> MSLHEKMQTDYLWVKDHSQADSWAKARTHGYNYIAHTVPNKKERYEMIWRSMGKSTDWELEKFRLGKKFPDRGNKRRWFKNLFRLIKNPMGYIFWKTYKARLAKPSLIVTSMFIGFTLGFIKLKAQSIAY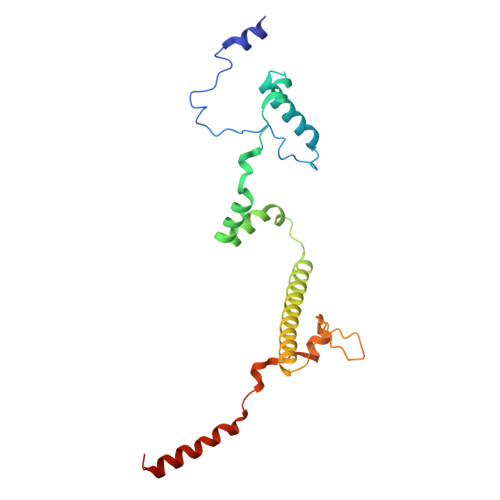SKKQYATLRAGKNIEGSGQVHFGYHDQKWGMPAIPMFQLMYYELPGNSIVVNPCRNQNYRLYFEMRKKLGILPA> SHHHHHHSSGLVPRGSHMTSSNDISLASKDPTTFPLGCSPDITTPKKGLSMELYSYDFRKKGSYPCWDAAYLDPN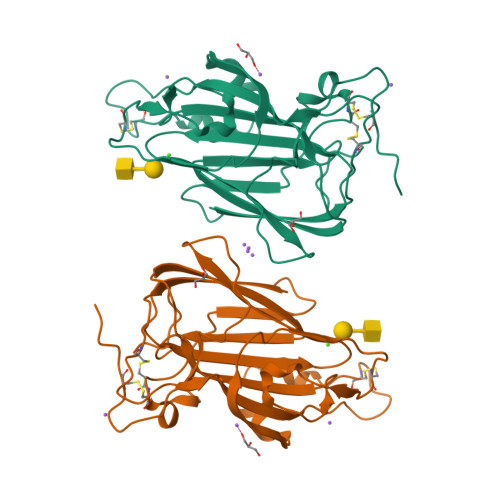YPRTGYKSHRLLAKVDGVTGNINFYYHATKGCTPQLGHLPASYNYPKPLTMTNFTMLLYGYFRPKVTGFHTFTISADDLLFVNFGAGNAFDCCRRDSSADHFGNYQAYAIWGSKTAKDELTVHLDAGVYYPIRLFYNNREYDGALSFTFKTESNENTVSDFSEYFFSLDDTEEGCPGLISYDSS> FPTIPLSRLFQNAMLRAHRLHQLAFDTYEEFEEAYIPKEQKYSFLQAPQASLCFSESIPTPSNREQAQQKSNLQLL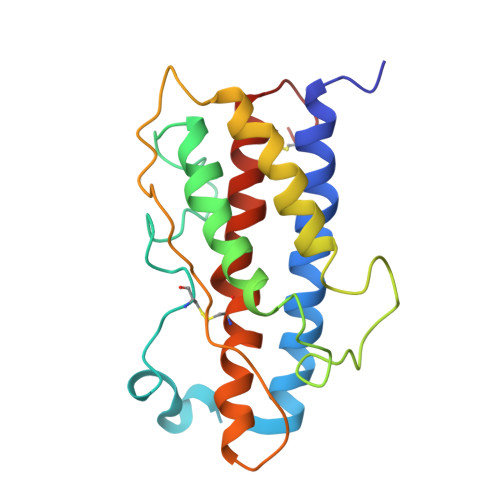RISLLLIQSWLEPVGFLRSVFANSLVYGASDSDVYDLLKDLEEGIQTLMGRLEDGSPRTGQAFKQTYAKFDANSHNDDALLKNYGLLYCFRKDMDKVETFLRIVQCRSVEGSCGF> MLSLDNYSYVHNITTQTNIDLSSQQTIHLASINGKGYIIFLRFFCEGSSACFTNVKFSVKANGLVLYSFRYIQLLELGQAIATAIPSSSQGFSTLLSNYNVLISSPIGTLPQLTLYDSYDNRYGAMLQPAFPLPFVNTLSLDV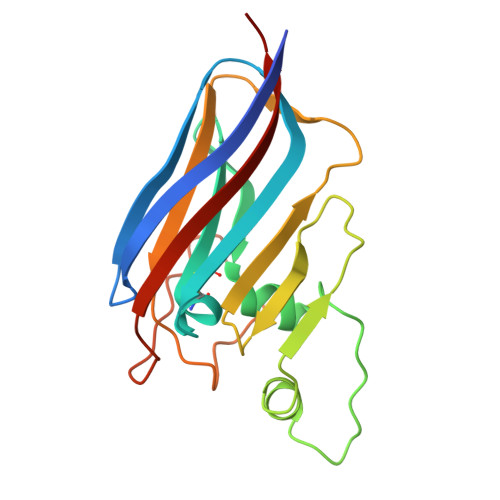DILPVSQSSYDPIPYSLNDNQISTNAPTGKGNISIEYLLYNCLV> MAIFDHQIKNVDKGNVVAILGAQWGDEGKGKIIDMLSEYSDITCRFNGGANAGHTISVNDKKYALHLLPCGVLYDNNISVLGNGMVIHVKSLMEEIESVGGKLLDRLYLSNKAHILFDIHQIIDSIQETKKLKEGKQIGTTKRGIGPCYSTKASRIGIRLGTLKNFENFKNMYSKLIDHLMDLYNITEYDKEKELNLFYNYHIKLRDRIVDVISFMNTNLENNKKVLIEGANAAMLDIDFGTYPYVTSSCTTVGGVFSGLGIHHKKLNLVVGVVKSYLTRVGCGPFLTELNNDVGQYLREKGHEYGTTTKRPRRCGWLDIPMLLYVKCINSIDMINLTKLDVLSGLEEILLCVNFKNKKTGELLEKGCYPVEEEISEEYEPVYEKFSGWKEDISTCNEFDELPEN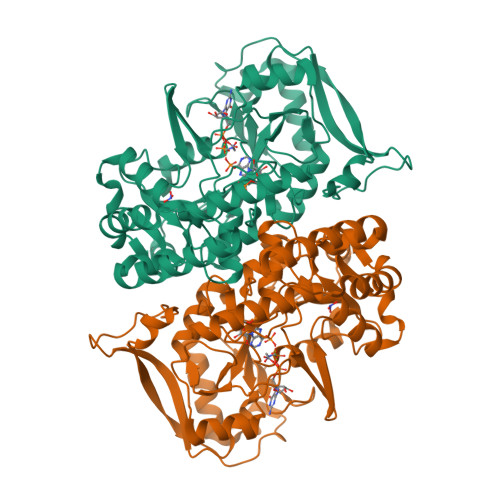AKKYILAIEKYLKTPIVWIGVGPNRKNMIVKKNFNLN> MDQDSLSSSLKTCYKYLNQTSRSFAAVIQALDGEMRNAVCIFYLVLRALDTLEDDMTISVEKKVPLLHNFHSFLYQPDWRFMESKE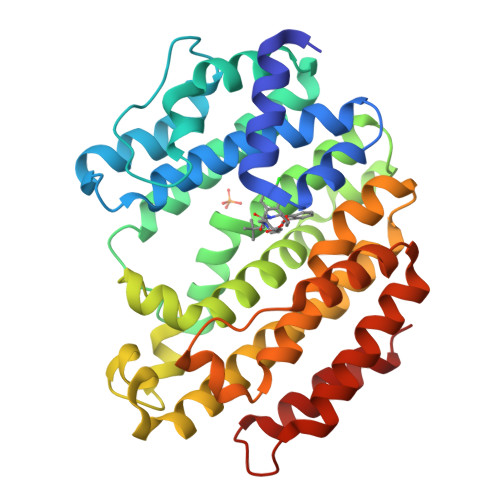KDRQVLEDFPTISLEFRNLAEKYQTVIADICRRMGIGMAEFLDKHVTSEQEWDKYCHYVAGLVGIGLSRLFSASEFEDPLVGEDTERANSMGLFLQKTNIIRDYLEDQQGGREFWPQEVWSRYVKKLGDFAKPENIDLAVQCLNELITNALHHIPDVITYLSRLRNQSVFNFCAIPQVMAIATLAACYNNQQVFKGAVKIRKGQAVTLMMDATNMPAVKAIIYQYMEEIYHRIPDSDPSSSKTRQIISTIRTQN> GSHMNRATQSIERSHR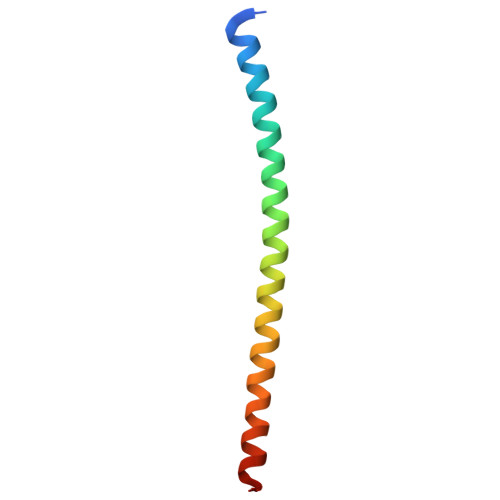IATETDQIGTEIIEELGEQRDQLERTKSRLVNTNENLSKSRKILRSMSR1-(2-azanylpyrimidin-4-yl)-6-[2-(1-oxidanylcyclohexyl)ethynyl]indole-3-carboxamide | C21 H21 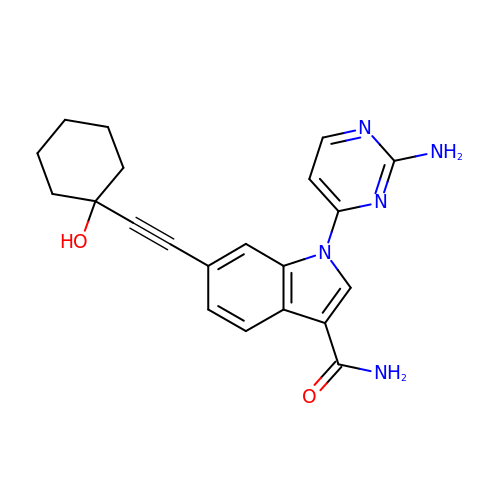N5 O2 | SXXLXIJRUAJXGS-UHFFFAOYSA-N> MEN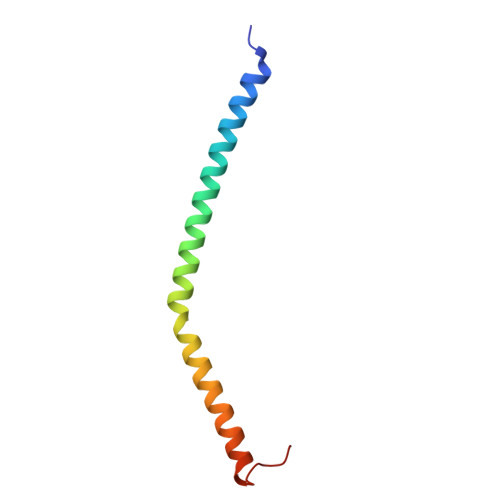PHEQVQANILSRIIGNVKRLNESVAILNQELVTINNRNKNLEIMGAICDNYHSSVQFNLEATNNKKPPL>[5x]GGVEVLEVKTGVDAITEVECFLNPEMGDPDENLRGFSLKLSAQNDFSSDSPERKMLPCYSTARIPL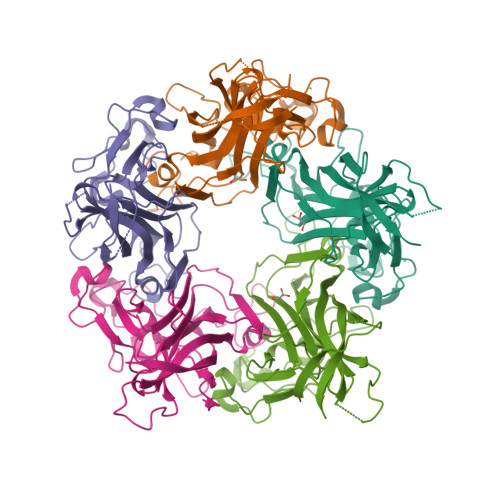PNLNEDLTSGNLLMWEAVTVQTEVIGITSMLNLHAGSQKVHEHGGGKPIQGSNFHFFAVGGEPLEMQGVLMNYRSKYPDGTITPKNPTAQSQVMNTDHKAYLDKNNAYPVECWVPDPSRNENARYFGTFTGGENVPPVLHVTNTATTVLLDEQGVGPLCKADSLYVSAADICGLFTNSSGTQQWRGLARYFKIRLRKRSVKNPYP> NQVLVPNLNPTPENLEVVGDGFKITSSINLVGEEEADENAVNALREFLTANNIEINSENDPNSTTLIIGEVDDDIPELDEALNGTTAENLKEEGYALVSNDGKIAIEGK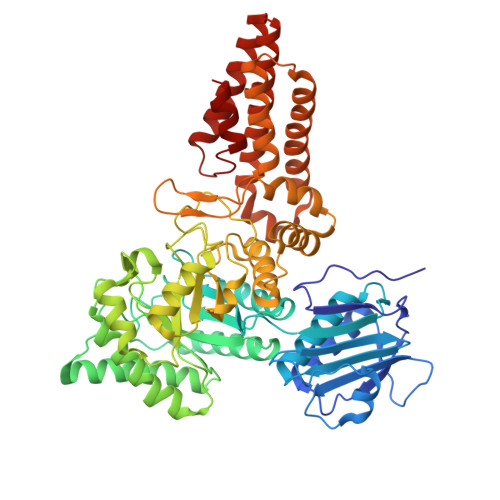DGDGTFYGVQTFKQLVKESNIPEVNITDYPTVSARGIVEGFYGTPWTHQDRLDQIKFYGENKLNTYIYAPKDDPYHREKWREPYPESEMQRMQELINASAENKVDFVFGISPGIDIRFDGDAGEEDFNHLITKAESLYDMGVRSFAIYWDNIQDKSAAKHAQVLNRFNEEFVKAKGDVKPLITVPTEYDTGAMVSNGQPRAYTRIFAETVDPSIEVMWTGPGVVTNEIPLSDAQLISGIYDRNMAVWWNYPVTDYFKGKLALGPMHGLDKGLNQYVDFFTVNPMEHAELSKISIHTAADYSWNMDNYDYDKAWNRAIDMLYGDLAEDMKVFANHSTRMDNKTWAKSGREDAPELRAKMDELWNKLSSKEDASALIEELYGEFARMEEACNNLKANLPEVALEECSRQLDELITLAQGDKASLDMIVAQLNEDTEAYESAKEIAQNKLNTALSSFAVISEKVAQSFIQEAL> MSEEAFIYEAIRTPRGKQKNGSLHEVKPLSLVVGLIDELRKRHPDLDENLISDVILGCVSPVGDQGGDIAR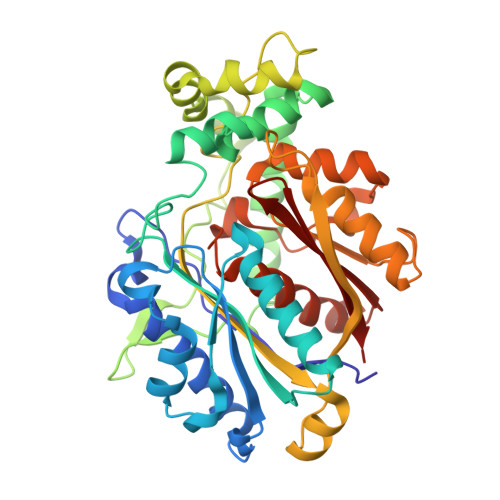AAVLASGMPVTSGGVQLNRFAASGLEAVNTAAQKVRSGWDDLVLAGGVESMSRVPMGSDGGAMGLDPATNYDVMFVPQSIGADLIATIEGFSREDVDAYALRSQQKAAEAWSGGYFAKSVVPVRDQNGLLILDHDEHMRPDTTKEGLAKLKPAFEGLAALGGFDDVALQKYHWVEKINHVHTGGNSSGIVDGAALVMIGSAAAGKLQGLTPRARIVATATSGADPVIMLTGPTPATRKVLDRAGLTVDDIDLFELNEAFASVVLKFQKDLNIPDEKLNVNGGAIAMGHPLGATGAMILGTMVDELERRNARRALITLCIGGGMGVATIIERV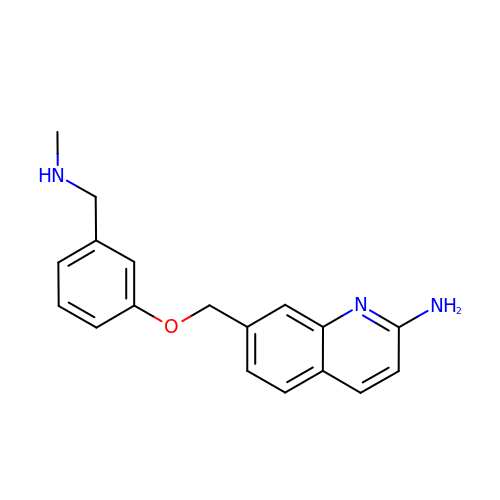7-[[3-(methylaminomethyl)phenoxy]methyl]quinolin-2-amine | C18 H19 N3 O | QFZGTQOWVVISDX-UHFFFAOYSA-N> GSHMAEGGGCRERPDAETQKSELGPLMRTTLQRGAQWYLIDSRWFKQWKKYVGFDSWDMYNVGEHNLFPGPIDNSGLFSDPESQTLKEHLI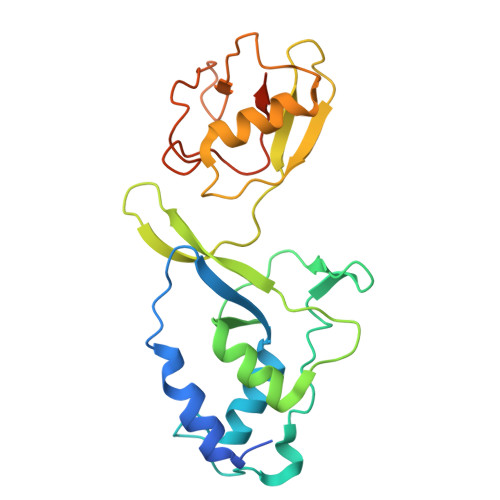DELDYVLVPTEAWNKLLNWYGCVEGQQPIVRKVVEHGLFVKHCKVEVYLLELKLCENSDPTNVLSCHFSKADTIATIEKEMRKLFNIPAERETRLWNKYMSNTYEQLSKLDNTVQDAGLYQGQVLVIEPQNEDGTWPRQTLQ>MVLYFIGLGLYDERDITVKGLEIAKKCDYVFAEFYTSLMAGTTLGRIQKLIGKEIRVLSREDVEMNFENIVLPLAKENDVAFLTPGDPLVATTHAELRIRAKRAGVESYVIHAPSIYSAVGITGLHIYKFGKSATVAYPEGNWFPTSYYDVIKENAERGLHTLLFLDIKAEKRMYMTANEAMELLLKVEDMKKGG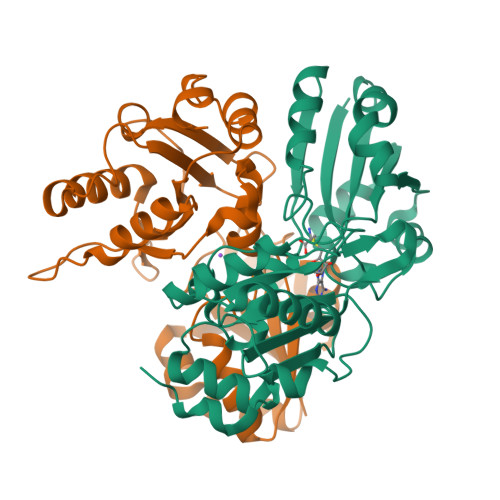VFTDDTLVVVLARAGSLNPTIRAGYVKDLIREDFGDPPHILIVPGKLHIVEAEYLVEIAGAPREILRVNV[2x]(3~{a}~{S},4~{R},5~{S},6~{R},7~{R},7~{a}~{R})-7-(hydroxymethyl)-2,2-bis(oxidanylidene)-3~{a},4,5,6,7,7~{a}-hexahydrobenzo[d][1,3,2]dioxathiole-4,5,6-triol 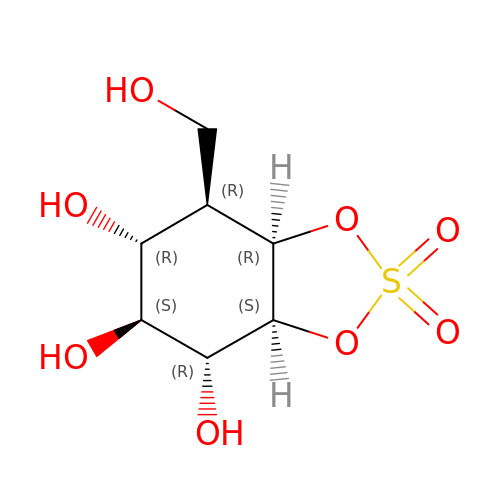| C7 H12 O8 S | ZCXRKCCKXOHKLN-GEGSFZHJSA-N> MKIILSGLALLASSVAAFAPQSIISANANNKNANVVLEAAKDDLIAIAEKSNPVLKYYDPLQLGSTTIWGETNSATIGFLRQSE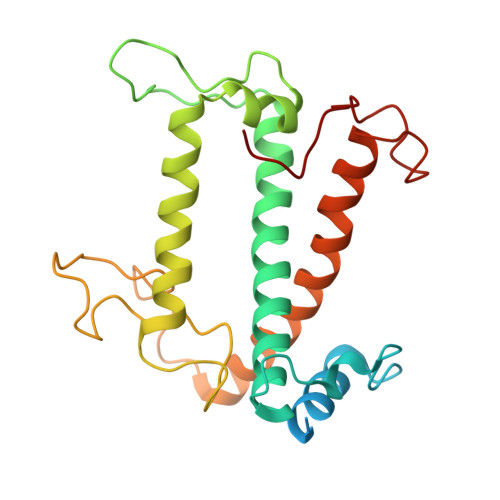IKHGRIAMAAFVGYIVQANGIHFPWPMSFDGTPFPADAGSPPEQWDALSDAAKWQIILFIGFLEWFSEAAGKHYMRGGKPGAFPNFSDSDLIPHPVPLNLYDPFGFSKGKTEAQKADGLIKELNNGRLAMIGIMGFLAEQKVEGSVPLLKGVVPHYDGEVMAPFM>[2x]MISKGFSTQTERINILKAQILNAKPCVESERAILITESFKQTEGQPAILRRALALKHILENIPITIRDQELIVGSLTKEPRSSQVFPEFSNKWLQDELDRLNKRTGDAFQISEESKEKLKDVFEYWNGKTTSELATSYMTEETREAVNCDVFTVGNYYYNGVGHVSVDYGKVLRVGFNGIINEAKEQLEKNRSIDPDFIKKEKFLNSVIISCEAAITYVNRYAKKAKEIADNTSDAKRKAELNEIAKICSKVSGEGAKSFYEACQLFWFIHAIIN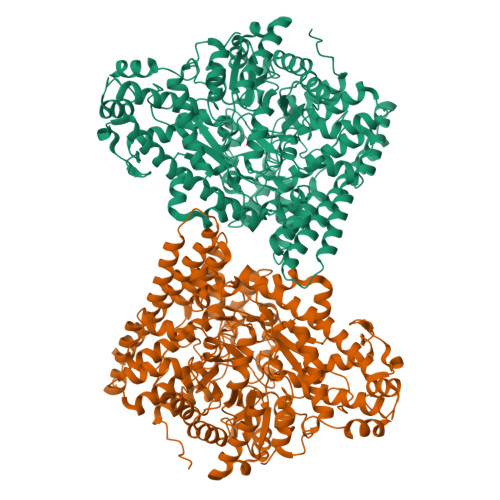IESNGHSISPARFDQYMYPYYENDKNITDKFAQELIDCIWIKLNDINKVRDEISTKHFGGYPMYQNLIVGGQNSEGKDATNKVSYMALEAAVHVKLPQPSLSVRIWNKTPDEFLLRAAELTREGLGLPAYYNDEVIIPALVSRGLTLEDARDYGIIGCVEPQKPGKTEGWHDSAFFNLARIVELTINSGFDKNKQIGPKTQNFEEMKSFDEFMKAYKAQMEYFVKHMCCADNCIDIAHAERAPLPFLSSMVDNCIGKGKSLQDGGAEYNFSGPQGVGVANIGDSLVAVKKIVFDENKITPSELKKTLNNDFKNSEEIQALLKNAPKFGNDIDEVDNLAREGALVYCREVNKYTNPRGGNFQPGLYPSSINVYFGSLTGATPDGRKSGQPLADGVSPSRGCDVSGPTAACNSVSKLDHFIASNGTLFNQKFHPSALKGDNGLMNLSSLIRSYFDQKGFHVQFNVIDKKILLAAQKNPEKYQDLIVRVAGYSAQFISLDKSIQNDIIARTEHVM> GPSGIVPQLQNIVSTVNLGCKLDLKTIALRARNAEYNPKRFAAVIMRIREPRTTALIFSSGKMVCTGAKSEEQSRLAARKYARVVQKLGFPAKFLDFKIQNMVGSCDVKFPIRLEGLVLTHQQFSSYEPELF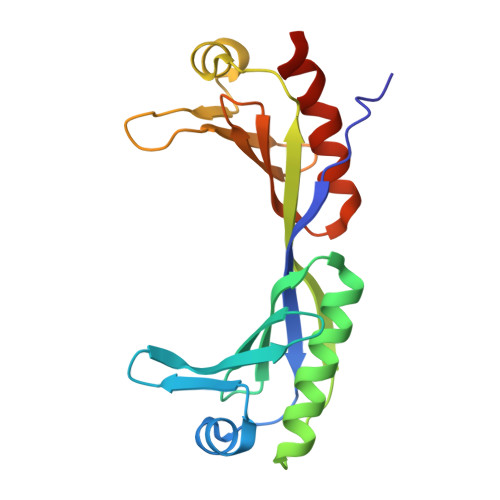PGLIYRMIKPRIVLLIFVSGKVVLTGAKVRAEIYEAFENIYPILKGFRKTT>[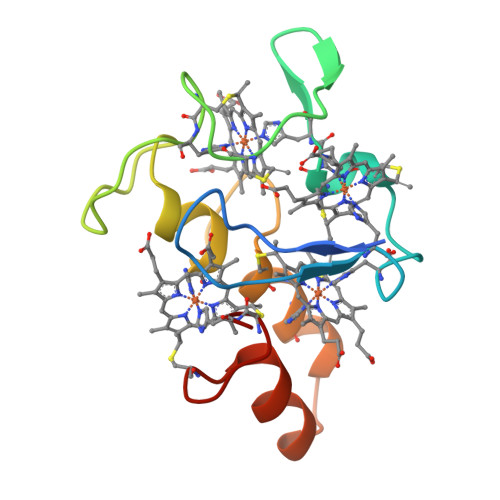2x]APKAPADGLKMEATKQPVVLNHSTHKSVKCGDCHHPVNGKEDYRKCGTAGCHDSMDKKDKSAKGYYHVMHDKNTKFKSCVGCHVEVAGADAAKKKDLTGCKKSKCHE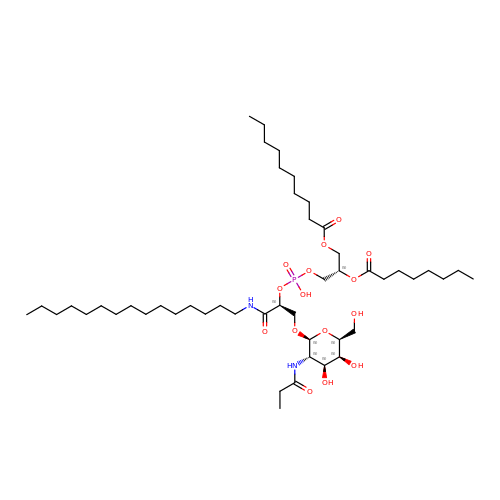[(2~{S})-3-[[(2~{S})-3-[(2~{S},3~{S},4~{S},5~{S},6~{S})-6-(hydroxymethyl)-4,5-bis(oxidanyl)-3-(propanoylamino)oxan-2-yl]oxy-1-oxidanylidene-1-(pentadecylamino)propan-2-yl]oxy-oxidanyl-phosphoryl]oxy-2-octanoyloxy-propyl] decanoate | C48 H91 N2 O15 P | BORXCJRMZBMSCX-GUINJWSRSA-N> MAFSRPGLPVEYLQVPSASMGRDIKVQFQGGGPHA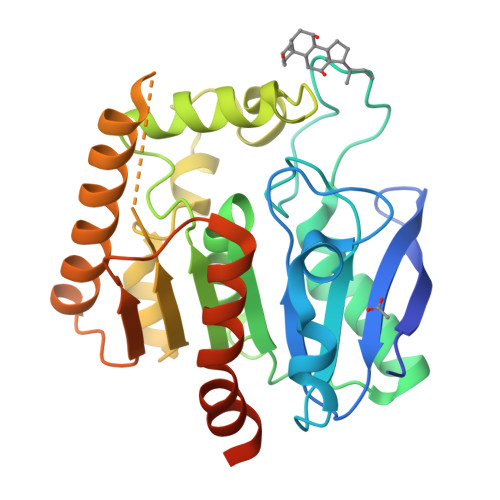VYLLDGLRAQDDYNGWDINTPAFEEYYQSGLSVIMPVGGQSSFYTDWYQPSQSNGQNYTYKWETFLTREMPAWLQANKGVSPTGNAAVGLSMSGGSALILAAYYPQQFPYAASLSGFLNPSEGWWPTLIGLAMNDSGGYNANSMWGPSSDPAWKRNDPMVQIPRLVANNTRIWVYCGNGTPSDLGGDNIPAKFLEGLTLRTNQTFRDTYAADGGRNGVFNFPPNGTQSWPYWNEQLVAMKADIQHVLNGATPPAAPAAPAAHHHHHH>[4x]MAQENLQKIVDSLESSRAEREELYKWFHQHPEMSMQEHETSKRIAEELEKLGLEPQNIGVTGQVAVIKNGEGPSVAFRADFDALPITENTGLDYSADPELGMMHACGHDLHTTALLGAVRALVENKDLWSGTFIAVHQPGEEGGGGARHMVDDGLAEKIAAPDVCFAQHVFNEDPAFGYVFTPGRFLTAASNWRIHIHGEGGHGSRPHLTKDPIVVAASIITKLQTIVSREVDPNEVAVVTVGSIEGGKSTNSIPYTVTLGVNTRASNDELSEYVQNAIKRIVIAECQAAGIEQEPEFEYLDSVPAVINDEDLTEQLMAQFREFFGEDQAVEIPPLSGSEDYPFIPNAWGVPSVMWGWSGFAAGSDAPGNHTDKFAPELPDALERGTQAILVAAAPWLMK

The skin glands secrete specific odourless precursor molecules, and the action of bacterial enzymes then triggers the release of the volatile odourants from these precursors. Precursor cleavage is then performed by an Nα-glutamine aminoacylase (N-AGA). We isolated this enzyme from a strain of Corynebacterium striatum that we had cultivated from axilla washings. The N-AGA enzyme releasing odouriferous acids has broad substrate specificity for the acyl part of the substrates, and a wide variety of Gln conjugates are secreted by the host and cleaved by this bacterial enzyme.

The availability of the N-AGA in pure form allowed a detailed characterization of this enzyme, and it was possible to resolve the crystal structure of the enzyme bound to the tetrahedral transition-state inhibitor at a resolution of 1.75 Å, which we report here for the first time. Thus, a highly selective transition-state inhibitor could be developed, that binds this enzyme with a Ki in the nanomolar range. This inhibitor contains the substructure of Gln, the non-cleavable phosphinic group, which mimics the tetrahedral transition state of the amide group and a large acyl part for high-affinity binding. In the crystal structure, two dimers associate to form a tetramer. Each metal-binding domain contains two zinc atoms and one molecule of the inhibitor bound to the active site. The two zinc atoms are tightly bound by three histidine residues (His-107, His-168 and His-370), and they are linked by a highly conserved Cys-reside (Cys-105) with the sulfur atom serving as a ligand for both zinc atoms. The tetrahedral phosphinic group of the ligand is bound via its two oxygen atoms to the two zinc atoms offering to both of them a fifth coordination partner and mimicking the transition state of the substrate being cleaved. The free carboxylate group of the Gln side chain is bound by a salt bridge to Arg-264 and by a hydrogen bond to Asn-251. On the other side, the hydrophobic part of the inhibitor resides in a large hydrophobic pocket formed by the side chains of Phe-170, Leu-335, Phe-185, Leu-186, His-168, Gly-337 and Met-354, excluding any water molecules. The hydrophobic part of the synthetic inhibitor is larger than the acyl part of most natural substrates, but still has ample space in this pocket explaining the low substrate specificity of the enzyme for the acyl residue, accommodating a wide range of natural and synthetic substrates.>MSLRIPRIYHPISLENQTQCYLSEDAANHVARVLRMTEGEQLELFDGSNHIYPAKIIESNKKSVKVEILGRELADKESHLKIHLGQVISRGERMEFTIQKSVELGVNVITPLWSERCGVKLDAERMDKKIQQWQKIAIAACEQCGRNIVPEIRPLMKLQDWCAENDGALKLNLHPRAHYSIKTLPTIPAGGVRLLIGSEG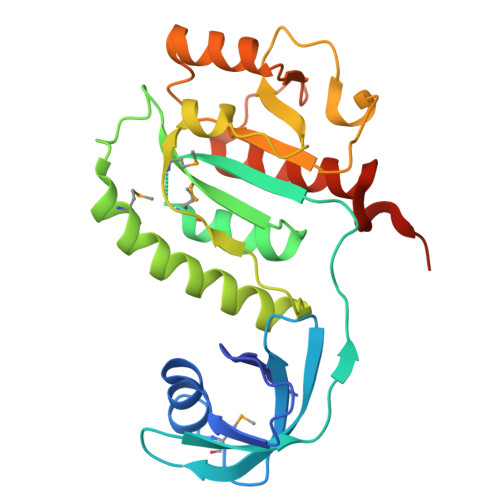GLSAQEIAQTEQQGFTEILLGKRVLRTETASLAAISALQICFGDLGEEGGSHHHHHH[2x]>[4x]DDIKVAVVGAMSGPIAQWGDMEFNGARQAIKDINAKGGIKGDKLVGVEYDDACDPKQA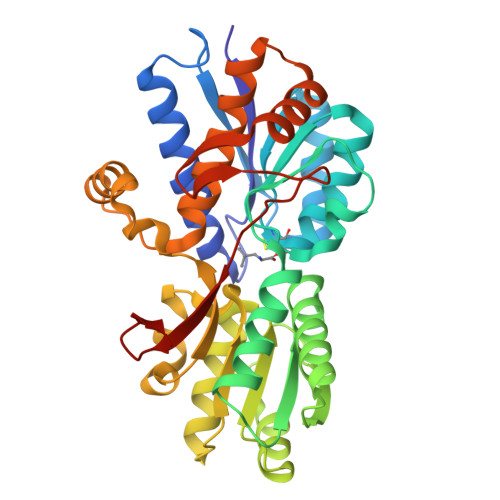VAVANKIVNDGIKYVIGHLCSSSTQPASDIYEDEGILMISPGATNPELTQRGYQHIMRTAGLDSSQGPTAAKYILETVKPQRIAIIHDKQQYGEGLARSVQDGLKAANANVVFFDGITAGEKDFSALIARLKKENIDFVYYGGYYPEMGQMLRQARSVGLKTQFMGPEGVGNASLSNIAGDAAEGMLVTMPKRYDQDPANQGIVDALKADKKDPSGPYVWITYAAVQSLATALERTGSDEPLALVKDLKANGANTVIGPLNWDEKGDLKGFDFGVFQWHADGSSTKAK>[4x]SNADSFIRQHLRKLAPYQPILPFEVLSSRLGRKPEDIVKLDANENPYGPPPEVMEALGSIRFPYVYPDPESRRLRAALAQDSGLESEYILVGCGADELIDLIMRCVLDPGDKIVDCPPTFTMYEFDAAVNGALVIKVPRRPDFSLNVEQIIEVVKQEKPKCIFLTSPNNPDGSIIDDDDLLKILELPILVVLDEAYIEFSTIESKMSWVKKHDNLIVLRTFSKRAGLAGLRVGYGAFPLSIIKYLWRAKQ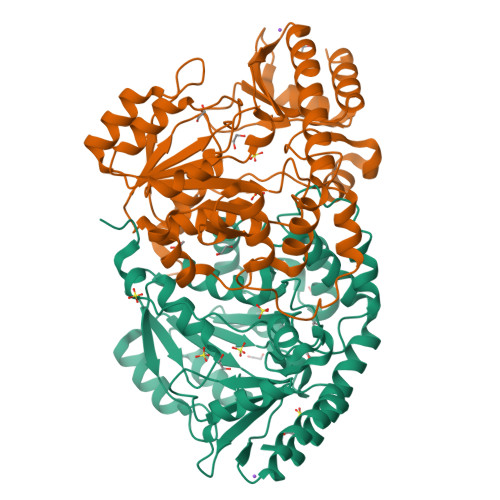PYNVSVAAEISACAALQNPTYLENVKDALVKERGRLFDLLKAVPFLKPFPSHSNFILCEVTSGVDPKKLKEDLAEMGVMIRHYSNKELKGYVRVSVGKPEHTDVLMNCISRLS Far upstream element (FUSE) binding protein 1 (FUBP1 or FBP1) is a multifunctional single-stranded DNA- (ssDNA) and RNA-binding protein, which acts as a master regulator of diverse cellular processes including transcription, mRNA stability and translation as well as RNA splicing. Central to its single-stranded nucleic acid (ssNA) interacting function of human FUBP1 is a tandem of four K homology (KH) motifs, namely KH1, KH2, KH3 and KH4, which is embedded in the middle region in between the self-regulatory and transactivation domains at the N- and C- termini, respectively. Comparison of the four structures showed that they all adopted an evolutionarily conserved eukaryotic KH-domain architecture, consisting of a three-stranded β-sheet packed on one side by three helices. A common property in recognition of up to four nucleotides is facilitated by a ‘minimal KH motif’ that constructs an ssNA hydrophobic binding cleft formed on one side by two short consecutive helices (α1 and α2) and the GXXG-motif-containing connecting loop and on the other side by the domain’s β-sheet and the variable loop that links the β2 and β3.

In addition, we observed also a unique, additional small α′ helix at the N-terminus of KH3. However, this structural element might be induced by the crystal packing as it existed only in one of the two molecules in the asymmetric unit. Of particular note was KH3, of which the short and compact β2-β3 variable loop and the presence of α1 R284 resulted in the more-enclosed, positively-charged binding groove, which was likely enabled also by the unique glycine-to-asparagine substitution in the GRNG motif at the upper part of the pocket. Since this motif was essential for ssDNA binding, we questioned whether this substitution might be a contributing factor to the distinctly stronger ssDNA-binding affinity observed for KH3. We therefore generated the KH3 mutant harbouring the GKGG motif resembling that of KH2 and KH4, and measured ssDNA binding using ITC. The results showed that the mutation did not exhibit an adverse effect, yet on a contrary slightly enhanced binding to ssDNA of ~ 1.7 fold was observed. This suggested therefore that the unique glycine-to-asparagine substitution was unlikely responsible for an increase in the nucleotide-binding affinity in KH3. As expected, in contrast to the wild type, all mutants did not show a shift in migration on native gels upon incubation with the selected ssDNA. These overall results suggested therefore that all four KH motifs of FUBP1 interacted with c-Myc FUSE ssDNA independently and individually, and KH1 and 3 might exert potential preference for ‘TTTGTGTT’ sequence while KH2 and KH4 might have broader binding specificity.

>[2x]SMFREVRNEYGSRIGGNEGIDVPIPRFAVGIVIGRNGEMIKKIQNDAGVRIQFKPDDGTTPERIAQITGPPDRCQHAAEIITDLLRSVQAGNP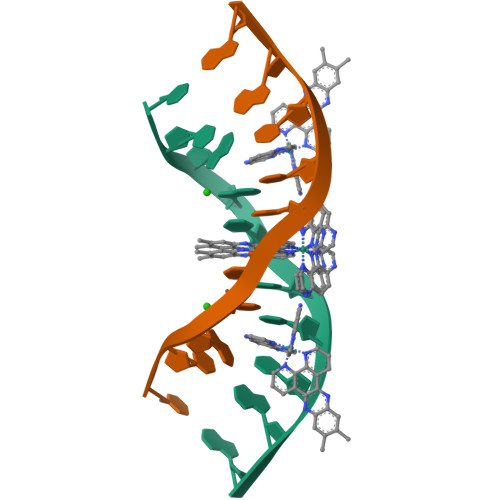> CCGGTACCGG>NAAEVIVYEHVNFGGKSFDATSDQPGAGDNLNDKISSIKVKSGTWRFYEYINYGGRYWDL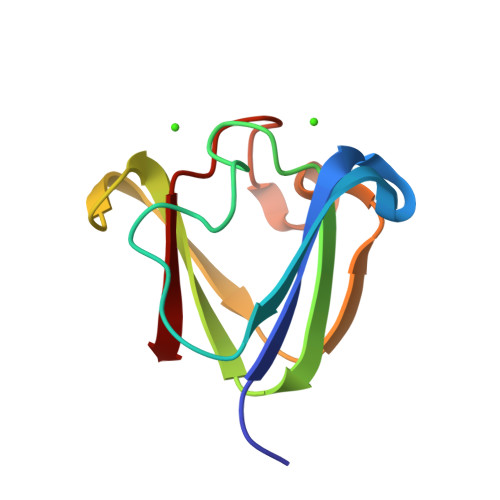GPGEYSSVESAGIPDNSISSFRQI[4x]~{N}-[3-[(2-fluorophenyl)sulfamoyl]phenyl]pyrazine-2-carboxamide 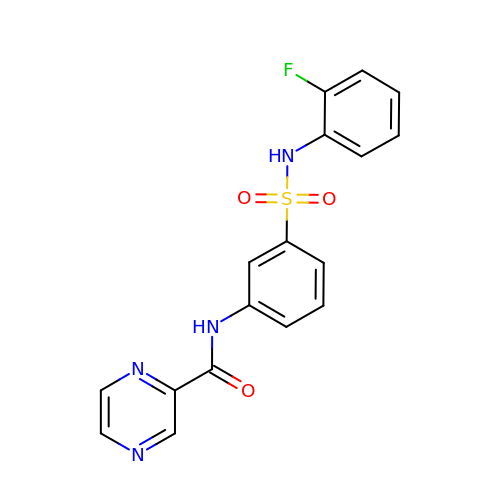| C17 H13 F N4 O3 S | ZTFLDPSGNNRWPL-UHFFFAOYSA-N> MRERPHTSGHHGAGE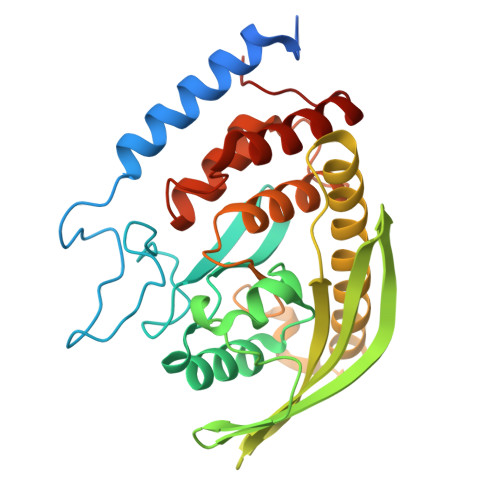ARATAPSTVSPYGPEARAELSSRLTTLRNTLAPATNDPRYLQACGGEKLNRFRDIQCRRQTAVRADLNANYIQVGNTRTIACQYPLQSQLESHFRMLAENRTPVLAVLASSSEIANQRFGMPDYFRQSGTYGSITVESKMTQQVGLGDGIMADMYTLTIREAGQKTISVPVVHVTTWPDFGVPESEVTKALASLVDQTAETKRNMYESKGSSAVADDSKLRPVIHCRAGVGRTAQLIGAMCMNDSRNSQLSVEDMVSQMRVQRNGIMVQKDEQLDVLIKLAEGQGRPLLNS> GSHHHHHHSQDPMPTPLPQLPSNVRDGENNVASTFLQAFFQLWDHDRLTLIPQFYDSETTFSVVFATDSPQDPASSSCSKFSRNLNILSPRHPSTLQRLFVGSNLIADLWKVLPATRHPSLDQTSQWLIDCHTFPHLADPTGMAPYAMGLMINVNGQCEEADISQNLYGTRTFSRCFILGPSKPGAPHPYRVLSDQLTLH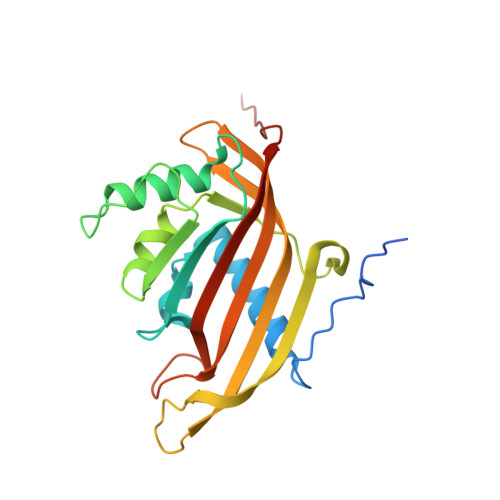TWKPQPAPQVGTV> AEAGITGTWYNQLGSTFIVT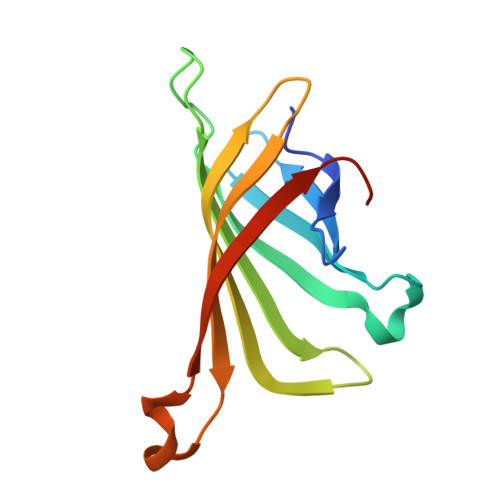AGADGALTGTYESAVGNAESRYVLTGRYDSAPATDGSGTALGWTVAWKNNYRNAHSATTWSGQYVGGAEARINTQWLLTSGTTEANAWKSTLVGHDTFTKVKPSAAS N-(1-acetyl-2,3-dihydro-1H-indol-4-yl)-3-chloro-2-hydroxybenzene-1-sulfonamide | C16 H15 Cl N2 O4 S | 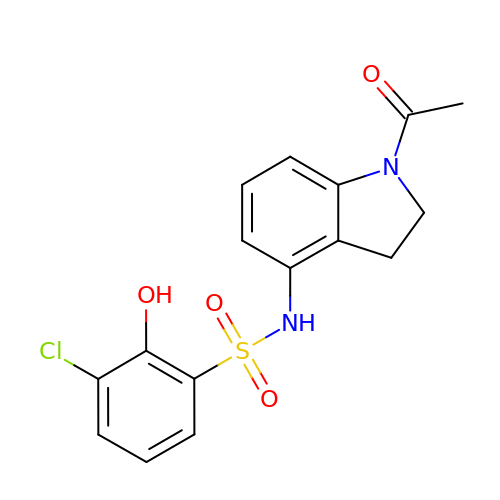OIXKKLRRYRMQMK-UHFFFAOYSA-N>MTHSLKALFALLFLYTAAVNAGV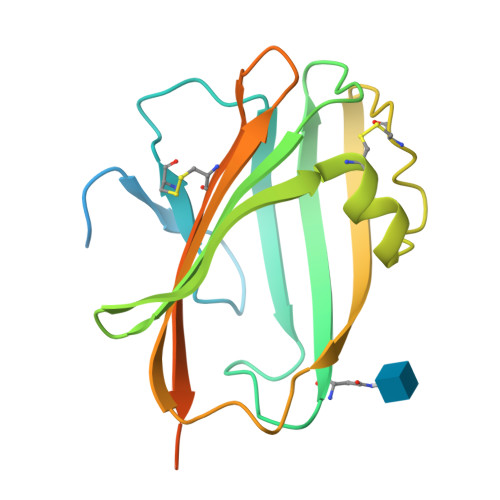IGIFNALPPPNTKPINGESPLYQCDILDKQLVEIKEVNLDPNPPVRGENLTISANGEVFETIEEGAYIDVEVRLGYIRLLSQTFDLCETLEDNDIEGLSCPIEPGEYNIKKIVEIPGEVPPGKYVVVARAYTEKDDLITCLTGEVIFPPRLVPRGSGGGGSGGGGSGGHHHHHHHHHH[3x]> MAHHHHHHMLKLIVETKTLVQSL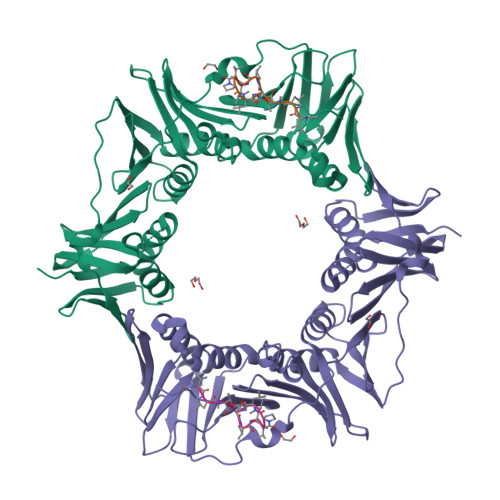GFARSVVEKRNVIPEYANIKLSAKDGNLELSSTNMDLYLSQKIAVQVLSEGEITVSTQTLSDIVRKLPDSELTLTELDIMKLEIKGQNCQFNLFTLPVSSFPAMDSIKPEVSFKISCADFAKIIESTKFSISLDETRYNLNGIYLHIKDKEFFAASTDGHRLSISWITLEEKIKNFGVILPQKSAEEILKIVKDLKNIHEDIEILLSSNKIKFICNENTILLSKLIDGTFPDYSAFIPKSSISKLVINRKIFADSIERIAIITVEKFRAIKLSLSRKTLEISAVGEARGNAKEIITASQDKESFYEYNCDESLVIGFNPQYLEDVLKAVKSNLVELYFSDISASAPVLIKFPQNPKDIFVIMPVKV;> XVPTLPLVPXG alpha-D-glucopyranosyl 6-O-sulfo-alpha-D-glucopyranoside | C12 H22 O14 S | 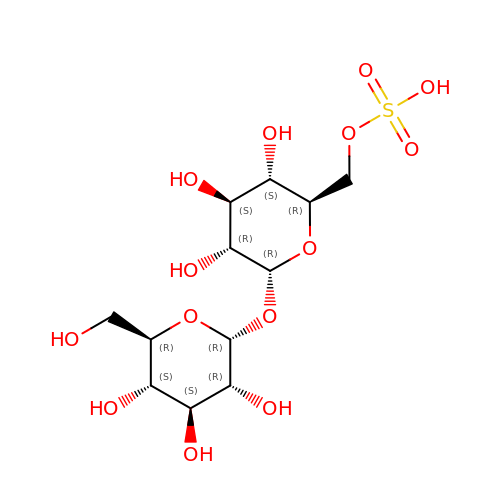AJWOGPXMZBTABG-LIZSDCNHSA-N> DNGLELS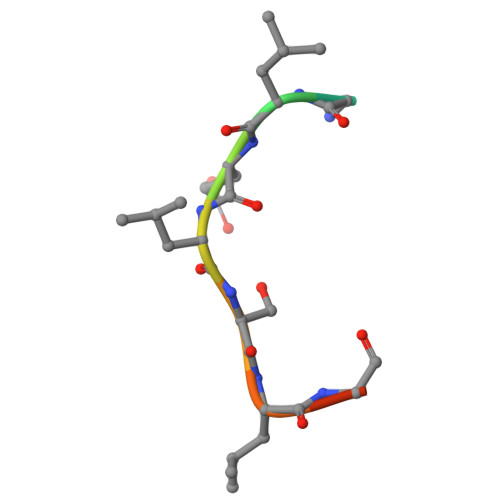LGLS N2-[(BENZYLOXY)CARBONYL]-N1-[(3S)-1-CYANOPYRROLIDIN-3-YL]-L-LEUCINAMIDE 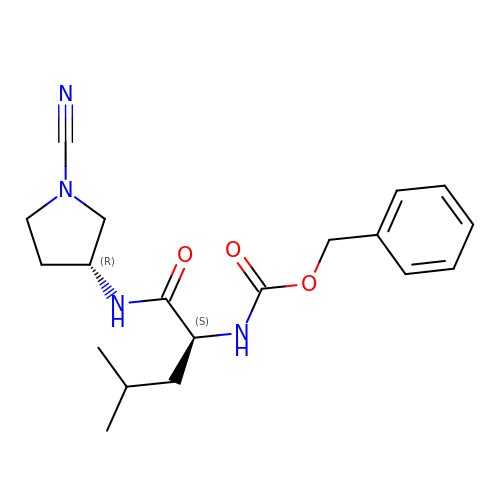| C19 H26 N4 O3 | IMTUSTXBVIALBC-SJORKVTESA-N> DQKLNTDLQETFSGFQKQLQSVLETDFFRDDSLMKGAIQMIHSKIMQMLLQSLIPEGLHQDITTDTGSKKSEIRSSDAHRILDLTWKHVHYPIFKYFQNWRNRNVAEGSRPNYAGHRQLNSILQKIFPQIHKLYYSTLELIFANYNLTALIPSDTRSKLNISTKKLNDDASNVLKPEDSFSIDCVMASQRCLLYIGCSQRYKIIMEHLSDRYQQADFQKPLRYLDIASTIVPSVGETFLQRGICYTHTKNFGNAAYQFVRSSLSRLPSDAGIPNFTNLLGDPNGSLFKKLLNSLDDLKVQETIKKRIINMEIME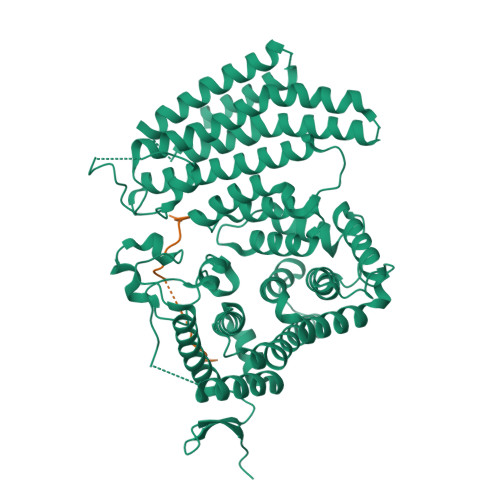FYILPLIGSHIFPQTWKNNRHSDRLKHFQTLLFDKIEIRYIKNISMIFQDLILLIGSFHMYQMINGVSSNIRSIQSETKFLEFIFKFFTHLIDKVIMKEFKNCEMFQYLAMARIMMCWIKSHKNVLKFAHRSTSFCQSMVNLTNELLSSNDLSISFEHLHRPTRDYFYEEDIMLKEFGPTKFTLSDFNDEKLLSMDNLPDRLVGKSKNKLTAKEEHSSRVQVLVYSNKKFLEKNCCGFKLDTEKKRYVHTAVK;> IVNPLFQLGLQREVNNDSFNEFDSQT5-ETHYL-2-PHENOXYPHENOL | C14 H14 O2 | 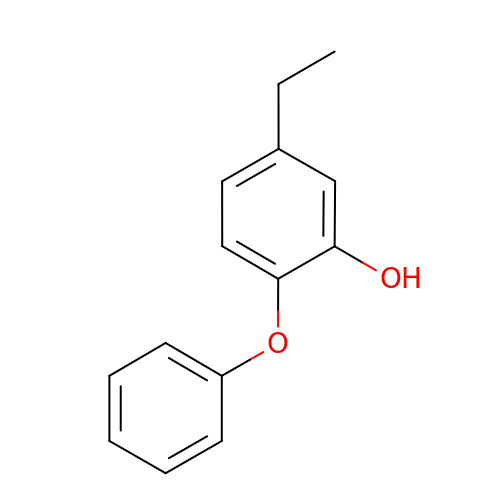XZOPHRPAUNJURP-UHFFFAOYSA-N>[4x]ISEFEKGYQSQLYTEMVGINNISKQFILKNPLDDNQ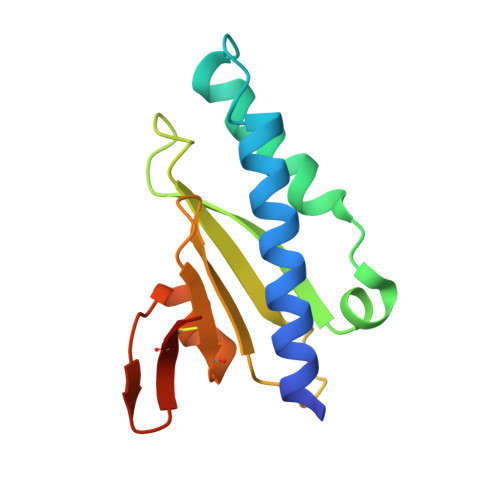TIKSKLERFVSGYKMNPKIAEKYNVSVHFVNKEKPRAYSLVGVPKTGTGYTLSVWMNSVGDGYKCRDAASARAHLETLSSDVGCEAFSNRKK The breakdown of the biaryl core was initiated by the ortho-hydroxylation of the substrate to yield 2,3-dihydroxybiphenyl (23DHBP). This aromatic hydroxylation was later attributed to a class “A” FPMO, 2-hydroxybiphenyl 3-monooxygenase (HbpA), which was isolated and characterised. Mechanistic studies confirmed that HbpA shared many of the catalytic characteristics of class “A” FPMOs such as PHBH. The monomer of HbpA broadly resembles the class “A” FPMO aromatic hydroxylases PHHY, RebC and RdmE of established structure and consists of three domains: an FAD nucleotide binding domain (D1) containing residues 4–76, 96–197 and 295–374; a “middle” domain (D2), composed of residues 77–95, 375–427 and 198–294; and a C-terminal domain (D3) incorporating a thioredoxin-like fold formed from residues 428–585. In this report, using a new genetic construct and exploiting advances in X-ray data collection time, we have used single crystals of HbpA to determine its structure in two forms: an FAD-bound form that allows characterisation of the active site, and an apo form that, although lacking flavin, gives extra information on the location of residues and structure of mobile loops that are absent from the FAD complex.

Although lacking the FAD coenzyme, the apo structure of HbpA has proved useful in providing information on secondary structural elements and residues that are missing from the FAD-complex structure. In the apo form, the amino acid backbone was complete from residues Ser4 to Arg228, Ala239 to Trp254 and Glu268 to Arg565. In the apo structure, the backbone Cα atoms of Arg242 and Met243 on strand β15 in D2 closest to FAD, for example, each move 2.5 Å away from the binding site in a superimposition of the two structures. The relative shift in domains is coincident with an absence of some electron density in regions in the FAD complex compared to the apo structure. These include density for the loop 195–203 that connects domains D1 and D2 as well as additional loops between the seven β-strands of domain D2, including region 245–249 between β15 and β16 and region 213–219 between β13 and β14, which features the short helix α8 in the apo structure. The reasons for the mobility of these loops on FAD binding are unclear; they correspond neither to substrate entry channels—as proposed, for example, for RdmE —nor to the region of the protein that would move as a result of FAD moving to the “out” position, as also observed in RdmE. The structural reorganisation upon FAD binding is also manifested in the orientation of the loop between residues 36 and 49 between β2 and β3, which moves to accommodate the isoalloxazine ring of FAD. In HbpA, helix α11 forms one side of a hydrophobic channel, the opening of which also includes the mobile loop 195–203, as revealed by the apo structure. The mobility in this region of the protein could mean that it serves as a gateway in HbpA for entry of the aromatic substrate.

>MSNSAETDVLIVGAGPAGAMSATLLASLGIRSLMINRWRSTSPGPRSHIINQRTMEILRDIGLEESAKSLAVPKEYMGEHVYATSLAGEEFGRIPAWASHPQAHAEHELASPSRYCDLPQLYFEPMVVSEAALRGADVRFLTEYLGHVEDQDGVTARLLDHVSGAEYEVRAKYIIGADGAHSLVAQNAGLPFEGQMGIGDSGSINIEFSADLSSLCEHRKGDMYWMFRAGSGINGVGVAALRMIRPWNKWICVWGYEKSKGTPEITKEEAKKIIHEIIGTDEIPVEVGPISTWTINQQYAVRNTSGRVFCMGDAVHRHTPMGGLGLNTSVQDAYNLAWKLALVLKGQAAPTLLDSYDAERSPVAKQIVERAFKSLSTFPPVFEALSLPPAPTESEMAEALVRLKDASEEGAKRRAALRKAMDATIIGLGGGHGVELNQRYVSRAVFPDGTPDPGFVRDQEFFYQASTRPGAHLPHVWLTENQRRISTLDLCGKGRFTLLTGLSGAAWKHEAEQVSQSLGIELKVCVIGPGQEFVDTYGEYAKISEIGESGALLVRPDMFIAFRAKDASREGLEQLNVAVKSILGRA[4x]>[4x]ANPCCSNPCQNRGECMSTGFDQYKCDCTRTGFYGENCTTPEFLTRIKLLLKPTPNTVWYILTHFKGVWNIVNNIPFLRSLIMKYVLTSRSYLIDSPPTYNVHYGYKSWEAFSNLSYYTRALPPVADDCPTPMGVKGNKELPDSKEVLEKVLLRREFIPDPQGSNMMFAFFAQHFTHQFFKTDHKRGPGFTRGLGHGVDLNHIYGETLDRQHKLRLFKDGKLKYQVIGGEVYPPTVKDTQVEMIYPPHIPENLQFAVGQEVFGLVPGLMMYATIWLREHNRVCDILKQEHPEWGDEQLFQTSRLILIGETIKIVIEDYVQHLSGYHFKLKFDPELLFNQQFQYQNRIASEFNTLYHWHPLLPDTFNIEDQEYSFKQFLYNNSILLEHGLTQFVESFTRQIAGRVAGGRNV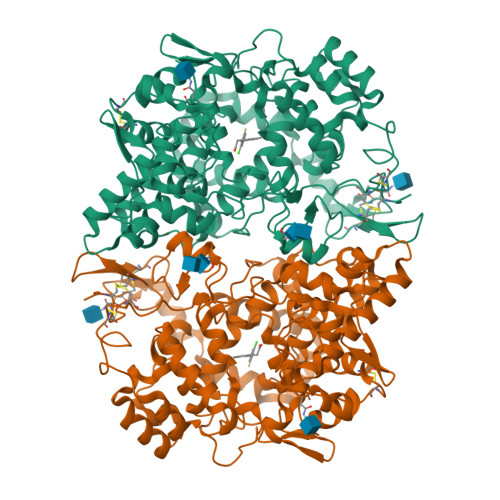PIAVQAVAKASIDQSREMKYQSLNEYRKRFSLKPYTSFEELTGEKEMAAELKALYSDIDVMELYPALLVEKPRPDAIFGETMVELGAPFSLKGLMGNPICSPQYWKPSTFGGEVGFKIINTASIQSLICNNVKGCPFTSFNVQDPQPTKTATINASASHSRLDDINPTVLIKRRSTEL(2~{R})-2-[[6-ethyl-5-(2-methylphenyl)thieno[2,3-d]pyrimidin-4-yl]amino]-3-phenyl-propanoic acid | C24 H23 N3 O2 S | 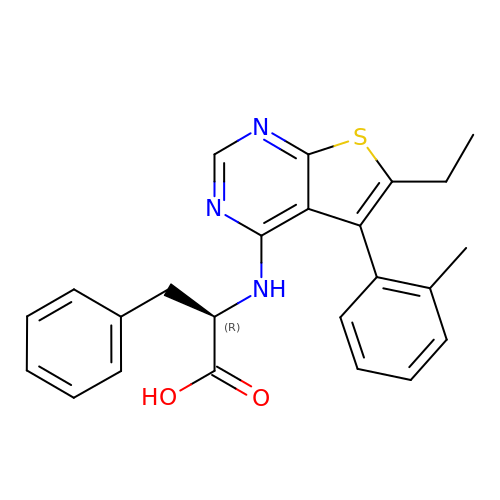BJYZTAWEBOABQO-GOSISDBHSA-N>QNACTLTAENHPSLTWSKCTSGGSCTSVQGSITIDANWRWTHRTDSATNCYEGNKWDTSYCSDGPSCASKCCIDGADYSSTYGITTSGNSLNLKFVTKGQYSTNIGSRTYLMESDTKYQMFQLLGNEFTFDVDVSNLGCGLNGALYFVSMDADGGMSKYSGNKAGAKYGTGYCDSQCPRDLKFINGEANVENWQSSTNDANAGTGKYGSCCSEMDVWEANNMAAAFTPHPCTVIGQSRCEGDSCGGTYSTDRYAGICDPDGCDFNSYRQGNKTFYGKGMTVDTTKKITVVTQFLKNSAGELSEIKRFYVQNGKVIPNS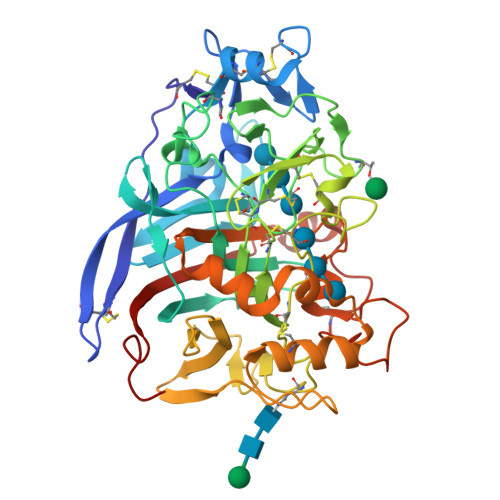ESTIPGVEGNSITQDWCDRQKAAFGDVTDFQDKGGMVQMGKALAGPMVLVMSIWDDHAVNMLWLDSTWPIDGAGKPGAERGACPTTSGVPAEVEAEAPNSNVIFSNIRFGPIGSTVSGLPDG[2x]>[2x]GHMDLKTAVFNAARDGKLRLLTKLLASKSKEEVSSLISEKTNGATPLLMAARYGHLDMVEFLLEQCSASIEVGGSVNFDGETIEGAPPLWAASAAGHLKVVQSLLNHGASVNNTTLTNSTPLRAACFDGHLEIVKYLVEHKADLEVSNRHGHTCLMISCYKGHKEIAQYLLEKGADVNRKSVKGNTALHDCAESGSLDIMKMLLMYCAKMEKDGYGMTPLL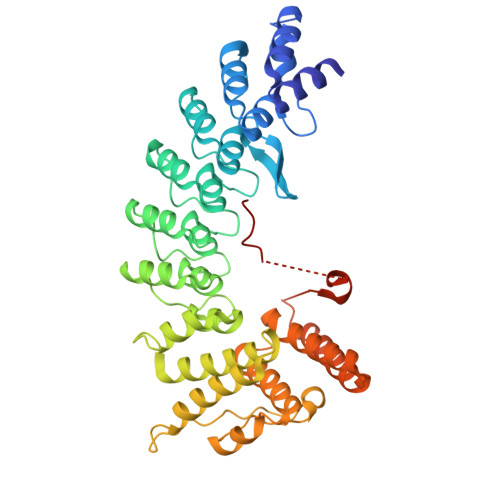SASVTGHTNIVDFLTHHAQTSKTERINALELLGATFVDKKRDLLGALKYWKKAMNMRYSDRTNIISKPVPQTLIMAYDYAKEVNSAEELEGLIADPDEMRMQALLIRERILGPSHPDTSYYIRYRGAVYADSGNFKRCINLWKYALDMQQSNLDPLSPMTASSLLSFAELFGGGSGGGSGGGSGGGSSVNSLLKELRG>[2x]SAA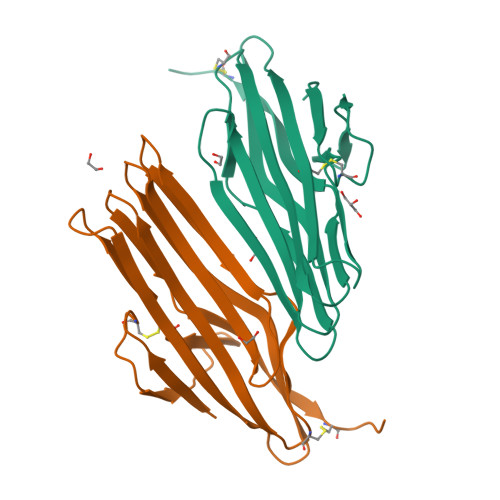AAGFVETAGNACEWTPGRYELSETEGRVRIPNGLYVKKEETSKIARGSCTFALTLKAPAGKKIVVRDSQQLISLRAYPQQTRVKAEVEIFKAGSQGAKQTLEIVAAEKAEKTTQYVGQKDVLLETACGGSDILRGNLSATIIGEGKGRAFAKNVTLDIQEVDCNLEHHHHHH> MASYKGLIVDVNGRSHENNLAHRTREIDRERLIVRRGQPFSITLQCSDSLPPKHHLELVLHLGKRDEVVIKVQKEHGARDKWWFNQQGAQD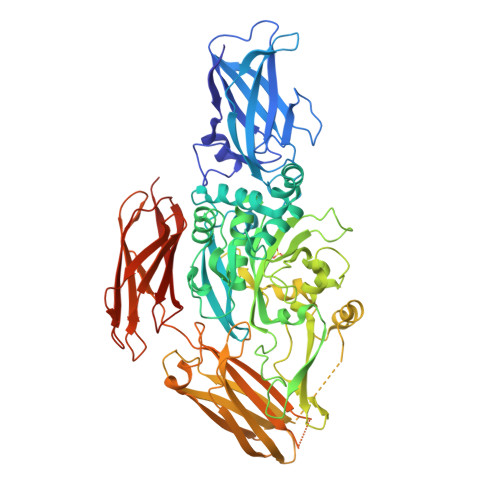EILLTLHSPANAVIGHYRLAVLVMSPDGHIVERADKISFHMLFNPWCRDDMVYLPDESKLQEYVMNEDGVIYMGTWDYIRSIPWNYGQFEDYVMDICFEVLDNSPAALKNSEMDIEHRSDPVYVGRTITAMVNSNGDRGVLTGRWEEPYTDGVAPYRWTGSVPILQQWSKAGVRPVKYGQCWVFAAVACTVLRCLGIPTRPITNFASAHDVDGNLSVDFLLNERLESLDSRQRSDSSWNFHCWVESWMSREDLPEGNDGWQVLDPTPQELSDGEFCCGPCPVAAIKEGNLGVKYDAPFVFAEVNADTIYWIVQKDGQRRKITEDHASVGKNISTKSVYGNHREDVTLHYKYPEGSQKEREVYKKAGRRVTEPSNEIAEQGRLQLSIKHAQPVFGTDFDVIVEVKNEGGRDAHAQLTMLAMAVTYNSLRRGECQRKTISVTVPAHKAHKEVMRLHYDDYVRCVSEHHLIRVKALLDAPGENGPIMTVANIPLSTPELLVQVPGKAVVWEPLTAYVSFTNPLPVPLKGGVFTLEGAGLLSATQIHVNGAVAPSGKVSVKLSFSPMRTGVRKLLVDFDSDRLKDVKGVTTVVVHKKYRSLITGLHTD8-[(3-Chloro-6,7,10,11-tetrahydro-9-methyl-7,11-methanocycloocta[b]quinolin-12-yl)amino]-N-(4-hydroxy-3-methoxybenzyl)octanamide 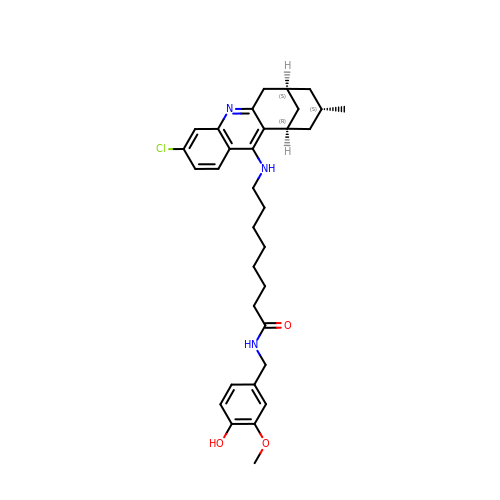| C33 H42 Cl N3 O3 | OMKWWMMJFOSSRE-OEMFJLHTSA-N>[2x]GAMGSGIHVQHIKRRDIVLKRELGEGAFGKVFLAECYNLSPTKDKMLVAVKALKDPTLAARKDFQREAELLTNLQHEHIVKFYGVCGDGDPLIMVFEYMKHGDLNKFLRAHGPDAMILVDGQPRQAKGELGLSQMLHIASQIASGMVYLASQHFVHRDLATRNCLVGANLLVKIGDFGMSRDVYSTDYYRVGGHTMLPIRWMPPESIMYRKFTTESDVWS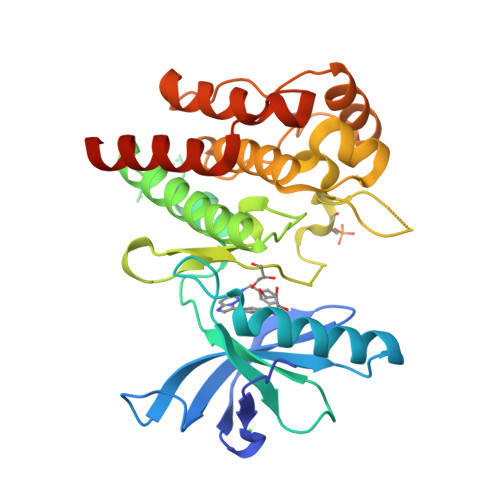FGVILWEIFTYGKQPWFQLSNTEVIECITQGRVLERPRVCPKEVYDVMLGCWQREPQQRLNIKEIYKILHALGKATPIYLDILG> MALKKAPKLFKTFFHWKLWKFSIIVFVFLVFLFLLQREVGVQDFKDEAGIEPVVGKKSHVLGLVLNAMNNIKGAKPKMQIKAPIRQTKVPGERHCLPGHYTPVELKPFLDRPLQDPNAPGASGKAFKTINLNSEEQKEKQAGEEKHCFNAFASDRISLHRDLGPDTRPPECIEQKFKRCPPLPTTSIIIVFHNEAWSTLLRTVHSVMYTSPAILLKEIILVDDASVDEYLHDKLDEYVKQFQIVKVVRQKERKGLITARLLGASVATGETLTFLDAHCECFYGWLEPLLARIAENPVAVVSPDIASIDLNTFEFSKPSPYGHSHNRGNFDWSLSFGWESLPKHENKRRKDETYPIRTPTFAGGLFSISKDYFEYIGSYDEEMEIWGGENIEMSFRVWQCGGQLEIMPCSVVGHVFRSKSPHTFPKGTQVITRNQVRLAEVWMDEYKEIFYRRNTEAAKIVKQKTFGDISKRIDLRQRLQCKNFTWYLSNVYPEAYVPDLNPLFSGYLKNIGNRMCLDVGENNHGGKPLIMYSCHGLGGNQYFEYSAHHEIRHN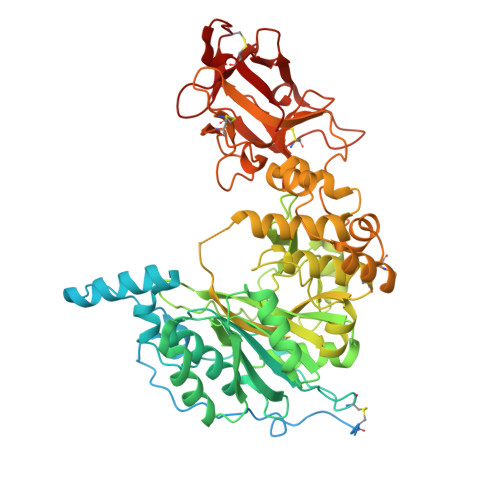IQKELCLHASKGPVQLRECTYKGQKTFAVGEEQWLHQKDQTLYNEALHMCLTGNGEHPSLASCNPSDPFQKWIFGQND> QDINAQLTTWFSQRLAGFSDEVVVTLRSSPNLLPSCEQPAFSMTGSAKLWGNVNVVARCANEKRYLQVNVQATGNYVAVAAPIARGGKLTPANVTLKRGRLDQLPPRTVLDIRQIQDAVSLRDLAPGQPVQLTMIRQAWRVKAGQRVQVIANGEGFSVNAEGQAMNNAAVAQNARVRMTSGQIVSGTVDSDGNILINLDP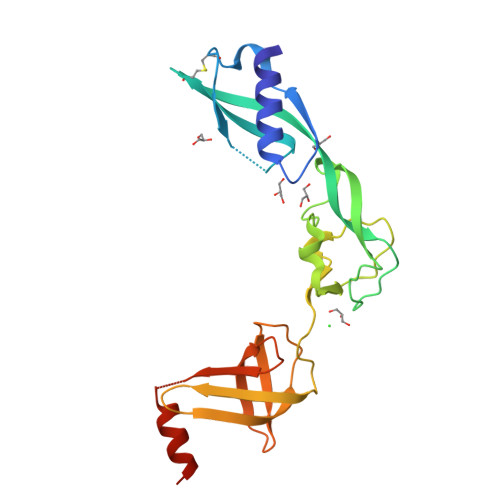NSSSVDKLAAALEHHHHHH> NLFQFAEMIVKMTGKNPLSSYSDYGCYCGWGGKGKPQDATDRCCFVHDCCYEKVKSCKPKLSLYSYSFQNGGIVCGDNHSCKRAVCECDRVAATCFRDNLNTYDKKYHNYP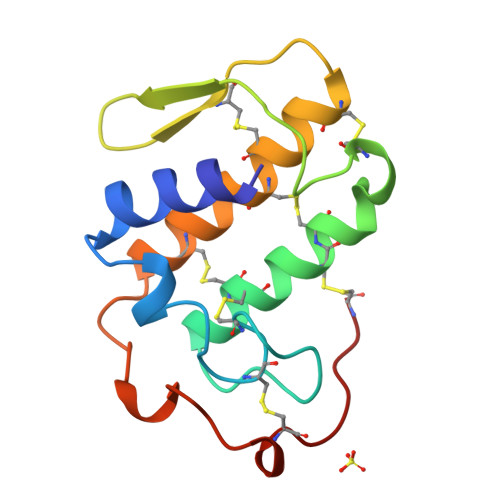PSQCTGTEQC>GSMASFEKFEPIFGEVVPERSDPGSGLLRRCLFHVYASDSYNLTVHVTDFISGVWTTILSVSQLDDMRDTVGIGGSWSEFVDYTVASLKSDNVKLLLGETSVSNGVKTARLVSQKAKGMPRINVPLTKMVESSASEAMANLSLELFRAFKSKQHLQGEVSFSAAATDEKDKRDATYNQL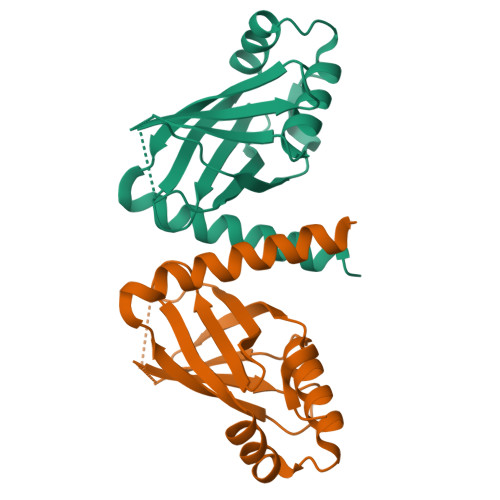ERYSRKLDVMAPSTNNRQDSPANQSAREANTKNPVKRVPAHRRTRKRGALLQDSEEEDG[10x]> AETTPWGQTFVGATVLSDSQAGNRTICIIDSGYDRSHNDLNANNVTGTNNSGTGNWYQPGNNNAHGTHVAGTIAAIANNEGVVGVMPNQNANIHIVKVFNEAGWGYSSSLVAAIDTCVNSGGANVVTMSLGGSGSTTTERNALNTHYNNGVLLIAAAGNAGDSSYSYPASYDSVMSVAAVDSNLDHAAFSQYTDQVEI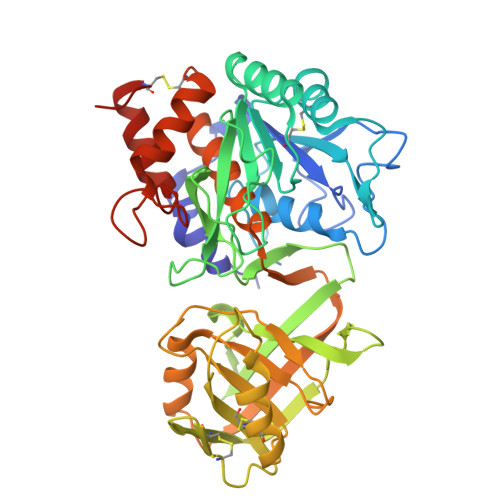SGPGEAILSTVTVGEGRLADITIGGQSYFSNGVVPHNRLTPSGTSYAPAPINASATGALAECTVNGTSFSCGNMANKICLVERVGNQGSSYPEINSTKACKTAGAKGIIVYSNSALPGLQNPFLVDANSDITVPSVSVDRATGLALKAKLGQSTTVSNQGNQDYEYYNGTSMATPHVSGVATLVWSYHPECSASQVRAALNATADDLSVAGRDNQTGYGMINAVAAKAYLDESCTGPTDPGTG Phylogenetic analysis shows that, within the rhodopsin superfamily, viral rhodopsins form a monophyletic family that consists of two distinct groups, VR1 and VR2. Here we present the results of a comprehensive structure-function study of two homologous proteins (61% sequence similarity) from the VR1 group, OLPVR1 (ADX06642.1), and VirChR1 (TARA-146-SRF-0.22-3-C376786_1). In this work, we demonstrate that VR1 rhodopsins are Na+/K+ selective light-gated ion channels that are inhibited by divalent cations. VirChR1s have proteorhodopsin-like architecture with short extracellular loops and share several structural features, such as membrane-associated ICL2 helix and an unconventional TM6-TM7 orientation.

Type B hexagonal crystals were grown at pH 7.0 using a monoolein (MO) lipid matrix, have the P1 space group, and contain two protein molecules in the asymmetric unit. Type A and type B crystals resulted in the obtaining of the OLPVR1 structures at the resolution of 1.4 and 1.6 Å, respectively. OLPVR1 molecules are nearly identical in both structures (root mean square deviation (RMSD) less than 0.2 Å), so hereafter, we refer to the structure from type A crystals as it has the highest resolution. The interfacial interaction in the putative dimer occurs mainly in the TM4 helix and involves several non-conservative residues, namely E108-E108’, Y111-Y111’, F122-F122’ with low surface interaction area (429 Å2). Strikingly different from other rhodopsins, the intracellular parts of TM6 and TM7 helices of OLPVR1 are significantly moved apart from each other far enough to form a pore. The pore is located at about 8 Å from the cytoplasmic side of the lipid membrane border and connects the inside of the protein with the groove on its surface, which leads further to the intracellular bulk. Surprisingly, in our structure, the groove and a part of the pore are occupied with a fragment of the lipid molecule, a host lipid of the crystallization matrix (MP and MO in case of 1.4 and 1.6 Å structures, respectively), which is likely to be a crystallization artifact and is discussed in more details in the Supplementary Notes.

>MDNIIMTAYISIFVQIITAIISVYGLFIPLNFKDIILREILILELIVQIIEFIFYIWLIITLQSINEDITYVRYFDWVLTTPVMLLTTVYFFEYMNSDDGIRKKEINDRDYVYLFYICLSNFFMLLIGYLGETKQINKMLTLFGGSFFLFLTFYLLYVKYTKENWMNYIVFYFMFLVWFLYGFAFMFPFSIKNQMYNILDIVSKNIYSIFIFIVILNQSYKLLLEHHHHHH[2x]>GPLGSHMGARNGRAGPSDSAFSFTKSRARVLTEAPKVTFKDVAGAEEAKEELKEIVEFLKNPSRFHEMGARIPKGVLLVGPPGVGKTHLARAVAGEARVPFITASGSDFVEMFVGVGAARVRDLFETAKRHAPCIVFIDEIDAVGRKRGSGVGGGNDEREQTLNQLLVEMDGFEKDTAIVVMAATNRPDILDPALLRPGRFDRQIAIDAPDVKGREQILRIHARGKPLAEDVDLALLAKRTPGFVGADLENLLNEAALLAAREGRRKITMKDLEEAADRVMMLPAKKSLVLSPRDRRITAYHEAGHALAAHFLEHADGVHKVTIVPRGRALGFMMPRREDMLHWSRKRLLDQIAVALAGRAAEEIVFDDVTTGAENDFRQATELARRMITEWGM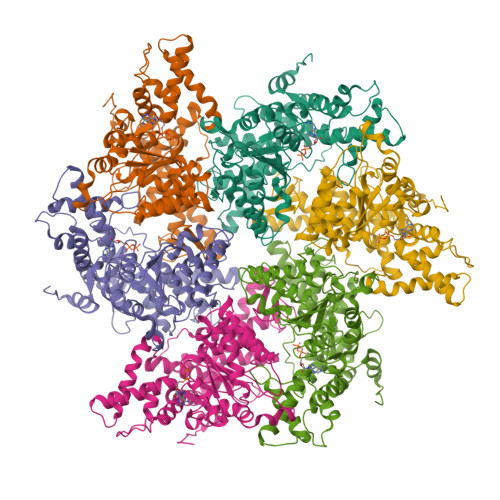HPEFGPVAYAVREDTYLGGYDVRQYSEETAKRIDEAVRRLIEEQYQRVKALLLEKREVLERVAETLLERETLTAEEFQRVVEGLPLEAPEEAREEREPPRVVPKVKPGGALGGA[6x]>[2x]GAMGSTPIELKGSSFTLSVVHLHEAEPKVIHQALEDKIAQAPAFLKHAPVVLNVSALEDPVNWSAMHKAVSATGLRVIGVSGCKDAQLKAEIEKMGLPILTEG

Proper cell division at the mid-site of gram-negative bacteria reflects critical regulation by the min system (MinC, MinD and MinE) of the cytokinetic Z ring, which is a polymer composed of FtsZ subunits. MinC and MinD act together to inhibit aberrantly positioned Z-ring formation. MinC consists of two domains: an N-terminal domain (MinCNTD), which interacts with FtsZ and inhibits FtsZ polymerization, and a C-terminal domain (MinCCTD), which interacts with MinD and inhibits the bundling of FtsZ filaments. MinC is a critical regulator of FtsZ polymerization that is bound to MinD and oscillates from one polar region within the cell to the other.

We targeted E. coli MinC (EcoMinC) for a structural study and determined the crystal structure of the dimeric EcoMinCNTD at 2.3 Å resolution. We observed EcoMinCNTD as a dimer within the asymmetric unit. EcoMinCNTD forms a dimer via domain swapping between the first β strands in each subunit, as observed in the StyMinCNTD structure. Dimerization of TmaMinC is mediated solely by the MinCCTD domain; MinCNTD is not involved in dimerization in this species. By contrast, TmaMinC lacks the corresponding Gly and Ser residues and hydrophobic residues that stabilize the domain swapped β1–β1 interaction. To generate monomeric EcoMinCNTD, this antiparallel β1–β1 interaction should be broken and the hydrophobic residues will become exposed, because the long β1 strand cannot fold back to make the β-hairpin structure, as observed in the structure of TmaMinCNTD. Thus we see dimeric EcoMinCNTD in the result of size-exclusion chromatography, in a broad range of protein concentrations, as well as in the EcoMinCNTD crystal structure. By using unfused-EcoMinCNTD, we observed that EcoMinCNTD forms a stable dimer in solution and in the crystal, enabling us to conclude that EcoMinC dimerizes through both EcoMinCCTD and Eco­MinCNTD. Taken together, the results of our structural study of EcoMinCNTD reveal that domain swapped dimerization is a likely mode of interaction with polymeric FtsZ.Clinical and environmental isolates of Stenotrophomonas maltophilia produce an enterobactin-like siderophore that promotes bacterial growth under low-iron conditions. In bacteria producing enterobactin-related molecules, EntB and its homologs are usually multi-domain proteins in which the amino portion acts as an isochorismatase and the carboxy domain serves as an aryl carrier protein (ArCP). However, in S. maltophilia the isochorismatase and ArCP functions are encoded by two distinct genes: entB and entB′, respectively. A crystal structure determination revealed EntB to be an unusual, single-domain form of isochorismatase enzyme.

The S. maltophilia EntB (SmEntB) structure was determined at 1.78 Å resolution. The protein core consists of a six-stranded parallel β-sheet (β3–β2–β1–β4–β5–β6). The cleft that is located between the lobe and the central core of the protein is part of the putative active site. Although a single chain is observed in the asymmetric unit, crystallographic symmetry revealed the presence of a dimer. Analytical size-exclusion chromatography estimated a molecular weight of 61.8 kDa, consistent with dimerization. In our structure, Gln79 and Arg88 interact with a formate, which occupies the same position as the ring carboxylate. Indeed, in SmEntB a water molecule is present in the same position, suggesting that the mechanism of substrate hydrolysis might be consistent with that proposed for VcVibB. Mapping the electrostatic potentials on the surface of SmEntB suggested that this putative isochorismate-binding site is mostly hydrophobic, but it is adjacent to charged residues. The hydrophobic residues of the pocket (Leu3, Phe42, Trp95, Tyr126, Tyr1552, Ile155 and Phe181) are conserved in SmEntB and other structural homologs, suggesting that isochorismate or other vinyl ethers may fit into the active site of SmEntB.

> SNAMALPRITDYPLPTAAELPQARGPWRPQRDRVALLVHDMQRYFLAAFDAGNAPLRPAVDNIARLLAHCRARGIPVFYTAQHGDQDRRDRGLQADLWGPGMRRSADHEPIIDALAPQPGEHVLVKHRYSAFQRSNLETLMRVRGRDQLLVTGVYAHIGCTATVVEAFQRDIEAFIAADAVADFSRADHDQALHWIARTSGVPMTTDQLLEVL>SEVEYR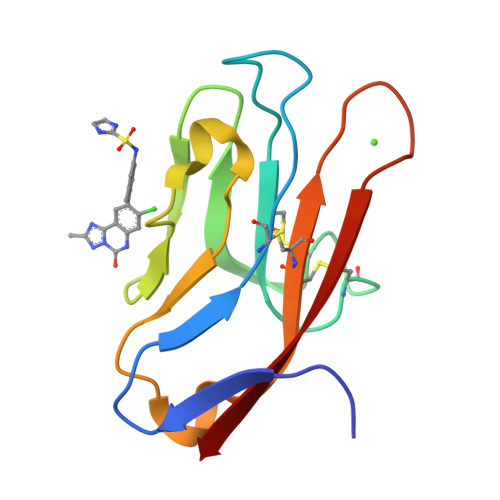AEVGQNAYLPCFYTPAAPGNLVPVCWGKGACPVFECGNVVLRTDERDVNYWTSRYWLNGDFRKGDVSLTIENVTLADSGIYCCRIQIPGIMNDEKFNLKLVIK[2x]> STMAIEKILTDAKTLLERLREHDAAAESLVDQSAALHRRVAAMREAGTALPDQYQEDASDMKDMS;> STMEQLSQYLQEALHREQMLEQKLATLQRLLAITQEASDTSWQALIDEDRLLSRLEVMGNQLQA

Our results supported a “two-arm” architecture of the STRIPAK complex, with the PP2Aa/c-bound STRNs acting as an organizing center to hold Hippo or other MST kinases with STRIP1 as one arm and SIKE1-SLMAP as the other. Moreover, we determined the crystal structures of the second coiled-coil domain of SIKE1 alone, and in complex with an STRN3 peptide, as well as the structure of the first coiled-coil domain of SIKE1 in complex with the first coiled-coil domain of SLMAP. SIKE1 functions to bridge SLMAP through CC1 on one hand and STRN3 through CC2 on the other. In particular, we discovered SIKE1 as a key adaptor that recruits MST-bound SLMAP to PP2A-bound STRN, forming a molecular arm MST-SLMAP-SIKE1-STRN-PP2Aa/c.

To further dissect at atomic level the SIKE1-SLMAP assembly, we determined the crystal structure of SIKE1 CC1 (residues 5–65) in complex with SLMAP CC1 (residues 167–226) at 2.3 Å resolution. An SIKE1 CC1 homodimer was interlaced with an SLMAP CC1 homodimer to assemble as a parallel four-helical bundle. A group of hydrophobic residues including I5, I8, A12, L15, L19, A26, L29, L36, V40, and M43 from SIKE1 CC1, and L168, L172, A175, L182, L186, L189, and L193 from SLMAP CC1 packed together to form a hydrophobic core. Moreover, residues D11, D23, Q32, and R39 from SIKE1 CC1 contacted residues Q173, R178, K185, Q190, S200, and D201 from SLMAP CC1 through hydrogen bonds and salt bridges. As shown in the bio-layer interferometry and MBP pulldown results, except for SIKE1-M43E, all other mutations on the complex interface including SIKE1 (L15D, L19D, L36D) and SLMAP (L182D, L186D, L189D, L193D) abolished the interactions between SIKE1 and SLMAP. Taken together, these results revealed a 2:2 heterotetrameric assembly of SIKE1-SLMAP and identified the leucine residues on the complex interface, namely L15, L19, and L36 of SIKE1 and L182, L186, L189, and L193 of SLMAP essential for SIKE1-SLMAP assembly. A further mapping experiment identified residues 5–65 of SIKE1 and residues 167–226 of SLMAP as the minimal regions mediating the interactions between the two proteins with a Kd of 6.9 μM. Meanwhile, SIKE1 CC1 can form a 2:2 hetrotetramer with SLMAP CC1. More importantly, SLMAP associated with STRN3 only in the presence of SIKE1. Together, these results indicated that SLMAP is recruited to STRN3 via SIKE1.>GPLGSLTASMLASAPPQEQKQMLGERLFPLIQAMHPTLAGKITGMLLEIDNSELLHMLESPESLRSKVDEAVAV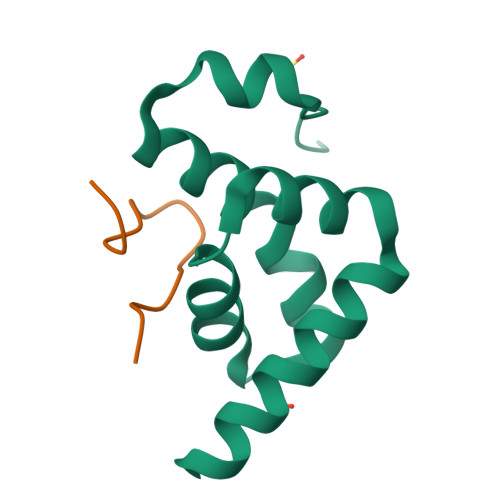LQAHQA[2x];>[2x]SINWPPEFHPGVPWKGLQ> AQPDIKFASKEYGVTIGESRIIYPLDAAGVMVSVKNTQDYPVLIQSRIYDENKEKESEDPFVVTPPLFRLDAKQQNSLRIAQAGGVFPRDKESLKWLCVKGIPPKDEDIWVDDATNKQKFNPDKDVGVFVQFAINNCIKLLVRPNELKGTPIQFAENLSWKVDGGKLIAENPSPFYMNIGELTF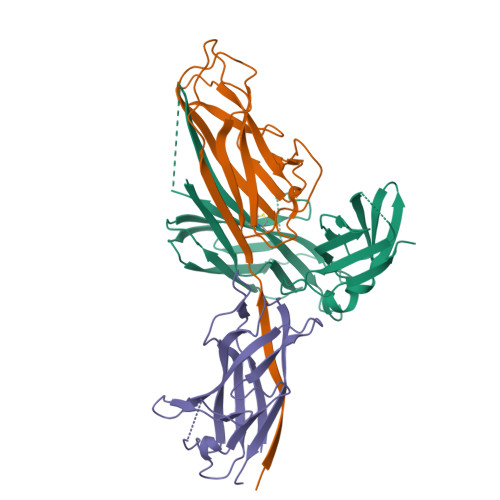GGKSIPSHYIPPKSTWAFDLPKGLAGARNVSWRIINDQGGLDRLYSKNVTL;>[2x]ADLTASTTATATLVEPARITLTYKEGAPITIMDNGNIDTELLVGTLTLGGYKTGTTSTSVNFTDAAGDPMYLTFTSQDGNNHQFTTKVIGKDSRDFDISPKVNGENLVGDDVVLATGSQDFFVRSIGSKGGKLAAGKYTDAVTVTVSNQ>SPKCIQCGQYLDDPDLKYGQHPPDAVDEPQMLTNEKLSIFDANESGFESYEALPQHKLTCFSVYCKHGHLCPIDTGLIEKNIELFFSGSAKPIYDDDPSLEGGVNGKNLGPINEWWITGFDGGEKALIGFSTSFAEYILMDPSPEYAPIFGLMQEKIYISKIVVEFLQSNSD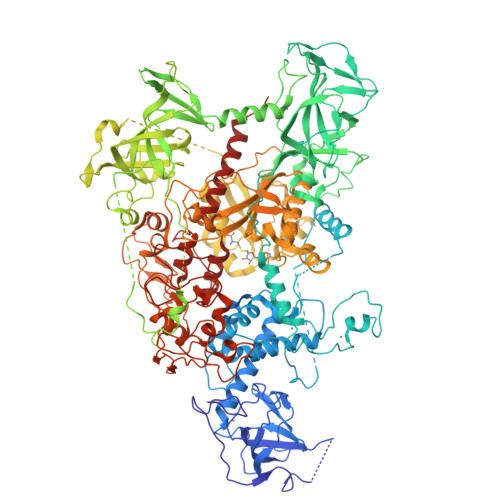STYEDLINKIETTVPPSGLNLNRFTEDSLLRHAQFVVEQVESYDEAGDSDEQPIFLTPCMRDLIKLAGVTLGQRRAQARRQTIRHSTREKDRGPTKATTTKLVYQIFDTFFAEQIEKDDREDKENAFKRRRCGVCEVCQQPECGKCKACKDMVKFGGSGRSKQACQERRCPNMAMKEADDDEEVDDNIPEMPSPKKMHQGKKKKQNKNRISWVGEAVKTDGKKSYYKKVCIDAETLEVGDCVSVIPDDSSKPLYLARVTALWEDSSNGQMFHAHWFCAGTDTVLGATSDPLELFLVDECEDMQLSYIHSKVKVIYKAPSENWAMEGGMDPESLLEGDDGKTYFYQLWYDQDYARFESPPKTQPTEDNKFKFCVSCARLAEMRQKEIPRVLEQLEDLDSRVLYYSATKNGILYRVGDGVYLPPEAFTFNIKLSSPVKRPRKEPVDEDLYPEHYRKYSDYIKGSNLDAPEPYRIGRIKEIFCPKKSNGRPNETDIKIRVNKFYRPENTHKSTPASYHADINLLYWSDEEAVVDFKAVQGRCTVEYGEDLPECVQVYSMGGPNRFYFLEAYNAKSKSFEDPPNHARSPGNKGKGKGKGKGKPKSQACEPSEPEIEIKLPKLRTLDVFSGCGGLSEGFHQAGISDTLWAIEMWDPAAQAFRLNNPGSTVFTEDCNILLKLVMAGETTNSRGQRLPQKGDVEMLCGGPPCQGFSGMNRFNSRTYSKFKNSLVVSFLSYCDYYRPRFFLLENVRNFVSFKRSMVLKLTLRCLVRMGYQCTFGVLQAGQYGVAQTRRRAIILAAAPGEKLPLFPEPLHVFAPRACQLSVVVDDKKFVSNITRLSSGPFRTITVRDTMSDLPEVRNGASALEISYNGEPQSWFQRQLRGAQYQPILRDHICKDMSALVAARMRHIPLAPGSDWRDLPNIEVRLSDGTMARKLRYTHHDRKNGRSSSGALRGVCSCVEAGKACDPAARQFNTLIPWCLPHTGNRHNHWAGLYGRLEWDGFFSTTVTNPEPMGKQGRVLHPEQHRVVSVRECARSQGFPDTYRLFGNILDKHRQVGNAVPPPLAKAIGLEIKLCMLAKALTRVW[2x]>GSSKKVGTLNRFTQALVIAYVIGYVCVYNKGYQDTDTVLSSVTTKVKGIALTNTSELGERIWDVADYIIPPQEDGSFFVLTNMIITTNQTQSKCAENPTPASTCTSHRDCKRGFNDARGDGVRTGRCVSYSASVKTCEVLSWCPLEKIVDPPNPPLLADAENFTVLIKNNIRYPKFNFNKRNILPNINSSYLTHCVFSRKTDPDCPIFRLGDIVGEAEEDFQIMAVRGGVMGVQIRWDCDLDMPQSWCVPRYTFRRLDNKDPDNNVAPGYNFRFAKYYKNSDGTETRTLIKGYGIRFDVMVFGQAGKFNIIPTLLNIGAGLALLGLVNVICDWIVLTFMKRKQHYKEQ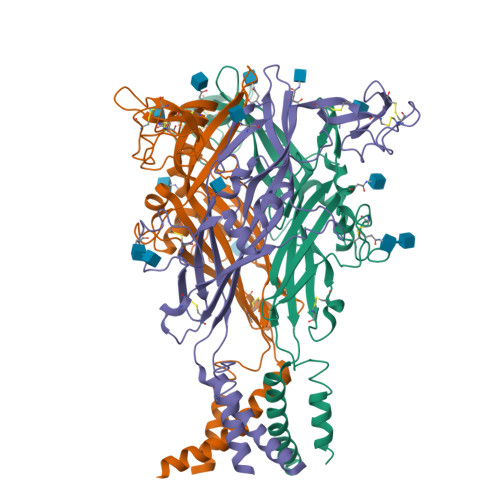KYTYVDDF[3x]>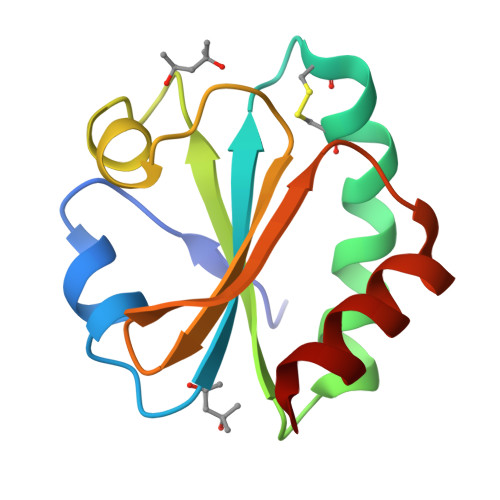[2x]SDKIIHLTDDSFDTDVLKADGAILVDFWAEWCGPCKMIAPILDEIAEEYQGKLTVAKLNIDQNPGTAPKYGIRGIPTLLLFKNGEVAATKVGALSKGQLKEFLDANLA>GFPIPDPYVWDPSFRTFYSIIDDEHKTLFNGIFHLAIDDNADNLGELRRCTGKHFLNQEVLMEASQYQFYDEHKKEHDGFINALDNWKGDVKWAKAWLVNHIKTIDFK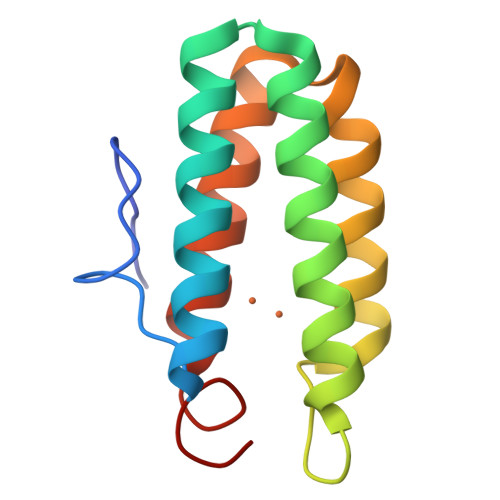YKGKI[2x]>[2x]MRGSHHHHHHGSAKNVVLDHDGNLDDFVAMVLLASNTEKVRLIGALCTDADCFVENGFNVTGKIMCLMHNNMNLPLFPIGKSAATAVNPFPKEWRCLAKNMDDMPILNIPENVELWDKIK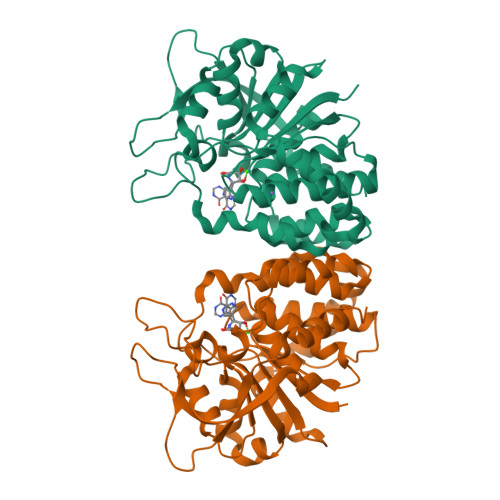AENEKYEGQQLLADLVMNSEEKVTICVTGPLSNVAWCIDKYGEKFTSKVEECVIMGGAVDVRGNVFLPSTDGTAEWNIYWDPASAKTVFGCPGLRRIMFSLDSTNTVPVRSPYVQRFGEQTNFLLSILVGTMWAMGGGYAWDALTAAYVVDQKVANVDPVPIDVVVDKQPNEGATVRTDAENYPLTFVARNPEAEFFLDMLLRSARAC>SNAGEVVDCHLSDMLQQLHSVNASKPSERGLVRQEEAEDPACIPIFWVSKWVDYSDKYGLGYQLCDNSVGVLFNDSTRLILYNDGDSLQYIERDGTESYLTVSSHPNSLMKKITLLKYFRNYMSEHLLKAGANITPREGDELARLPYLRTWFRTRSAIILHLSNGSVQINFFQDHTKLILCPLMAAVTYIDEKRDF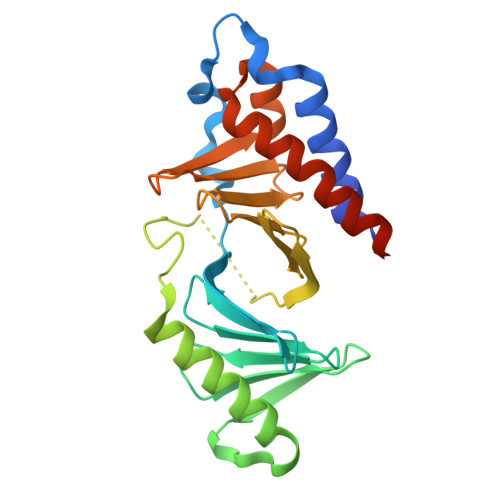RTYRLSLLEEYGCCKELASRLRYARTMVDKLLSSRSASNRLKAS[2x]>GPGSEFMGAWLRAIGLERYEEGLVHNGWDDLEFLSDITEEDLEEAGVQDPAHKRLLLDTLQLSKSSGENLYFQSSGSSGGSSGSEGVPFRTVSEWLESIKMQQYTEHFMVAGYTAIEKVVQMSNEDIKRIGVRLPGHQKRI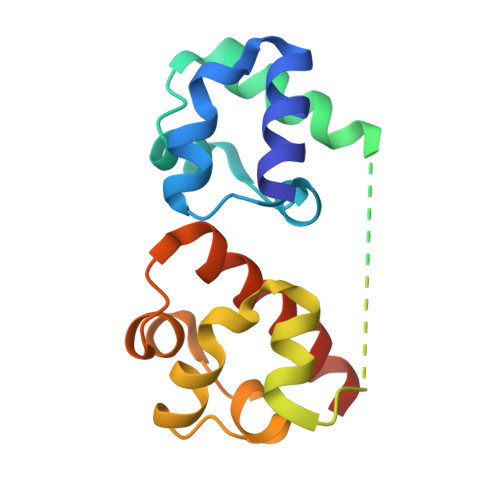AYSLLGLKDQVNTVGIPI[2x]> MTIHEHDRVSADRGGDSPHTTHALVDRLMAGEPYAVAFGGQGSAWLETLEELVSATGIETELATLVGEAELLLDPVTDELIVVRPIGFEPLQWVRALAAEDPVPSDKHLTSAAVSVPGVLLTQIAATRALARQGMDLVATPPVAMAGHSQGVLAVEALKAGGARDVELFALAQLIGAAGTLVARRRGISVLGDRPPMVSVTNADPERIGRLLDEFAQDVRTVLPPVLSIRNGRRAVVITGTPEQLSRFELYCRQISEKEEADRKNKVRGGDVFSPVFEPVQVEVGFHTPRLSDGIDIVAGWAEKAGLDVALARELADAILIRKVDWVDEITRVHAAGARWILDLGPGDILTRLTAPVIRGLGIGIVPAATRGGQRNLFTVGATPEVARAWSSYAPTVVRLPDGRVKLSTKFTRLTGRSPILLAGMTPTTVDAKIVAAAANAGHWAELAG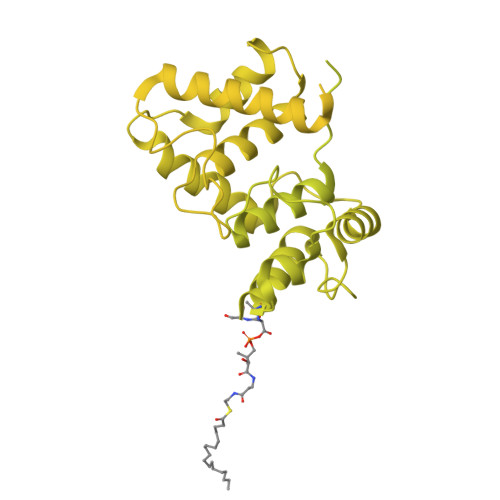GGQVTEEIFGNRIEQMAGLLEPGRTYQFNALFLDPYLWKLQVGGKRLVQKARQSGAAIDGVVISAGIPDLDEAVELIDELGDIGISHVVFKPGTIEQIRSVIRIATEVPTKPVIMHVEGGRAGGHHSWEDLDDLLLATYSELRSRANITVCVGGGIGTPRRAAEYLSGRWAQAYGFPLMPIDGILVGTAAMATKESTTSPSVKRMLVDTQGTDQWISAGKAQGGMASSRSQLGADIHEIDNSASRCGRLLDEVAGDAEAVAERRDEIIAAMAKTAKPYFGDVADMTYLQWLRRYVELAIGEGNSTADTASVGSPWLADTWRDRFEQMLQRAEARLHPQDFGPIQTLFTDAGLLDNPQQAIAALLARYPDAETVQLHPADVPFFVTLCKTLGKPVNFVPVIDQDVRRWWRSDSLWQAHDARYDADAVCIIPGTASVAGITRMDEPVGELLDRFEQAAIDEVLGAGVEPKDVASRRLGRADVAGPLAVVLDAPDVRWAGRTVTNPVHRIADPAEWQVHDGPENPRATHSSTGARLQTHGDDVALSVPVSGTWVDIRFTLPANTVDGGTPVIATEDATSAMRTVLAIAAGVDSPEFLPAVANGTATLTVDWHPERVADHTGVTATFGEPLAPSLTNVPDALVGPCWPAVFAAIGSAVTDTGEPVVEGLLSLVHLDHAARVVGQLPTVPAQLTVTATAANATDTDMGRVVPVSVVVTGADGAVIATLEERFAILGRTGSAELADPARAGGAVSANATDTPRRRRRDVTITAPVDMRPFAVVSGDHNPIHTDRAAALLAGLESPIVHGMWLSAAAQHAVTATDGQARPPARLVGWTARFLGMVRPGDEVDFRVERVGIDQGAEIVDVAARVGSDLVMSASARLAAPKTVYAFPGQGIQHKGMGMEVRARSKAARKVWDTADKFTRDTLGFSVLHVVRDNPTSIIASGVHYHHPDGVLYLTQFTQVAMATVAAAQVAEMREQGAFVEGAIACGHSVGEYTALACVTGIYQLEALLEMVFHRGSKMHDIVPRDELGRSNYRLAAIRPSQIDLDDADVPAFVAGIAESTGEFLEIVNFNLRGSQYAIAGTVRGLEALEAEVERRRELTGGRRSFILVPGIDVPFHSRVLRVGVAEFRRSLDRVMPRDADPDLIIGRYIPNLVPRLFTLDRDFIQEIRDLVPAEPLDEILADYDTWLRERPREMARTVFIELLAWQFASPVRWIETQDLLFIEEAAGGLGVERFVEIGVKSSPTVAGLATNTLKLPEYAHSTVEVLNAERDAAVLFATDTDPEPEPEEDEPVAESPAPDVVSEAAPVAPAASSAGPRPDDLVFDAADATLALIALSAKMRIDQIEELDSIESITDGAXSRRNQLLVDLGSELNLGAIDGAAESDLAGLRSQVTKLARTYKPYGPVLSDAINDQLRTVLGPSGKRPGAIAERVKKTWELGEGWAKHVTVEVALGTREGSSVRGGAMGHLHEGALADAASVDKVIDAAVASVAARQGVSVALPSAGSGGGATIDAAALSEFTDQITGREGVLASAARLVLGQLGLDDPVNALPAAPDSELIDLVTAELGADWPRLVAPVFDPKKAVVFDDRWASAREDLVKLWLTDEGDIDADWPRLAERFEGAGHVVATQATWWQGKSLAAGRQIHASLYGRIAAGAENPEPGRYGGEVAVVTGASKGSIAASVVARLLDGGATVIATTSKLDEERLAFYRTLYRDHARYGAALWLVAANMASYSDVDALVEWIGTEQTESLGPQSIHIKDAQTPTLLFPFAAPRVVGDLSEAGSRAEMEMKVLLWAVQRLIGGLSTIGAERDIASRLHVVLPGSPNRGMFGGDGAYGEAKSALDAVVSRWHAESSWAARVSLAHALIGWTRGTGLMGHNDAIVAAVEEAGVTTYSTDEMAALLLDLCDAESKVAAARSPIKADLTGGLAEANLDMAELAAKAREQMSAAAAVDEDAEAPGAIAALPSPPRGFTPAPPPQWDDLDVDPADLVVIVGGAEIGPYGSSRTRFEMEVENELSAAGVLELAWTTGLIRWEDDPQPGWYDTESGEMVDESELVQRYHDAVVQRVGIREFVDDGAIDPDHASPLLVSVFLEKDFAFVVSSEADARAFVEFDPEHTVIRPVPDSTDWQVIRKAGTEIRVPRKTKLSRVVGGQIPTGFDPTVWGISADMAGSIDRLAVWNMVATVDAFLSSGFSPAEVMRYVHPSLVANTQGTGMGGGTSMQTMYHGNLLGRNKPNDIFQEVLPNIIAAHVVQSYVGSYGAMIHPVAACATAAVSVEEGVDKIRLGKAQLVVAGGLDDLTLEGIIGFGDMAATADTSMMCGRGIHDSKFSRPNDRRRLGFVEAQGGGTILLARGDLALRMGLPVLAVVAFAQSFGDGVHTSIPAPGLGALGAGRGGKDSPLARALAKLGVAADDVAVISKHDTSTLANDPNETELHERLADALGRSEGAPLFVVSQKSLTGHAKGGAAVFQMMGLCQILRDGVIPPNRSLDCVDDELAGSAHFVWVRDTLRLGGKFPLKAGMLTSLGFGHVSGLVALVHPQAFIASLDPAQRADYQRRADARLLAGQRRLASAIAGGAPMYQRPGDRRFDHHAPERPQEASMLLNPAARLGDGEAYIG>[2x]GAMEVEVKLRLLTAAAHLRLTTLLTPYH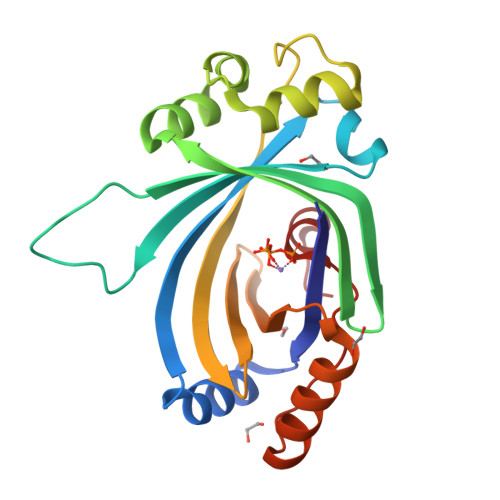LKTLHQRNTFFDTPKNDLSLRRAVLRLRFLQNAAVSAASPSPPRCIVSLKAKPTLANGISRVEEDEEEIEYWIGKECVESPAKLSDIGSRVLKRVKEEYGFNDFLGFVCLGGFENVRNVYEWRGVKLEVDETKYDFGNCYEIECETEEPERVKTMIEEFLTEEKIEFSNSDMTKFAVFRSGKLP>[4x]MAHHHHHHVGTGSNDDDDKSPDPNWELVYTARLQMVKVLAVLYDGGEHAKQVPGLLGTTENELGLRKWLEDQGHTLVTTSDKDREGSTFDRELEDAEII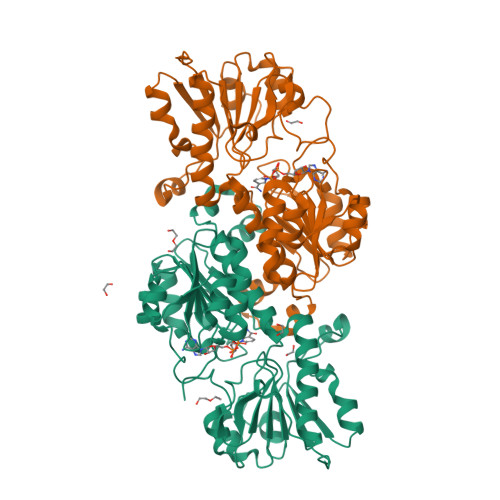ITTPFHPGYLTAERLARAKKLKLAVTAGIGSDHVDLDAANKTNGGITVAEVTGSCVVSVAEHVVMTILVLVRNFVPAHEQIEAGRWDVAEVAKDEYDLEGKVVGTVGVGRIGERVLRRLKGFDCKELLYYDYQPLSPEKEKEIGCRRVENLEEMLAQCDVVTINCPLHESTRGLFNKDLISKMKRGSWLVNTARGAIVVKEDVAEALRTGHLRGYGGDVWFPQPAPADHVLRTAKNPFGGGNAMVPHMSGTSLDAQKRYAEGVKRILDSYLSGRFDYRPEDLIVHQGKYATRAYGQREDVKIPGQHHHHHH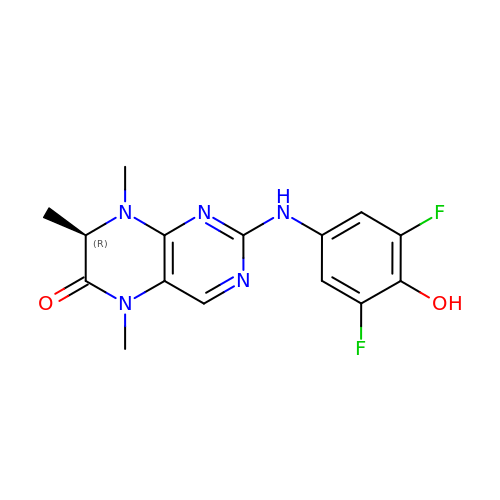(7R)-2-[(3,5-difluoro-4-hydroxyphenyl)amino]-5,7,8-trimethyl-7,8-dihydropteridin-6(5H)-one | C15 H15 F2 N5 O2 | GSJOYFAUMSHIJL-SSDOTTSWSA-N>[2x]MLPKDKLNPPTPSIYLENKRDAFFPPLHQFCTNPKNPV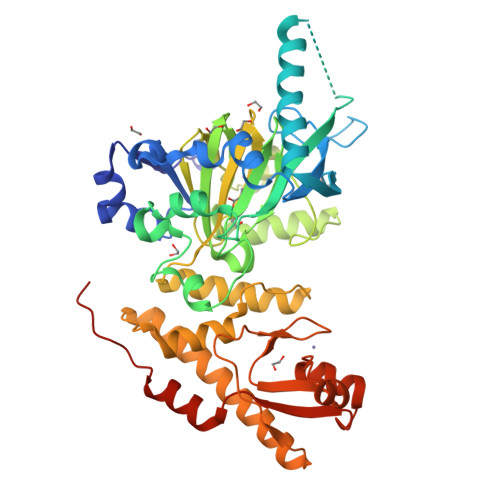TVIRGLAGALKLDLGLFSTKTLVEANNEHMVEVRTQLLQPADENWDPTGTKKIWRCESNRSHTTIAKYAQYQASSFQESLREENEKRTQHKDHSDNESTSSENSGRRRKGPFKTIKFGTNIDLSDNKKWKLQLHELTKLPAFARVVSAGNLLTHVGHTILGMNTVQLYMKVPGSRTPGHQENNNFCSVNINIGPGDCEWFVVPEDYWGVLNDFCEKNNLNFLMSSWWPNLEDLYEANVPVYRFIQRPGDLVWINAGTVHWVQAVGWCNNIAWNVGPLTACQYKLAVERYEWNKLKSVKSPVPMVHLSWNMARNIKVSDPKLFEMIKYCLLKILKQYQTLREALVAAGKEVIWHGRTNDEPAHYCSICEVEVFNLLFVTNESNTQKTYIVHCHDCARKTSKSLENFVVLEQYKMEDLIQVYDQFTLALSLSSSSAENLYFQ>[2x]MYDWFSEMRKKDPVYYDGNIWQVFSYRYTKEVLNNFSKFSSDLTGYHERLEDLRNGKIRFDIPTRYTMLTSDPPLHDELRSMSADIFS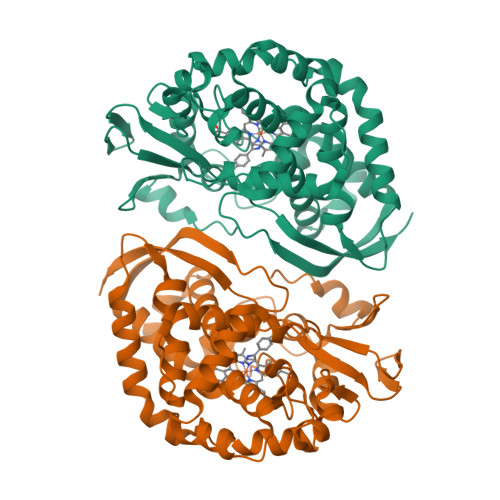PQKLQTLETFIRETTRSLLDSIDPREDDIVKKLAVPLPIIVISKILGLPIEDKEKFKEWSDLVAFRLGKPGEIFELGKKYLELIGYVKDHLNSGTEVVSRVVNSNLSDIEKLGYIILLLIAGNETTTNLISNSVIDFTRFNLWQRIREENLYLKAIEEALRYSPPVMRTVRKTKERVKLGDQTIEEGEYVRVWIASANRDEEVFHDGEKFIPDRNPNPHLSFGSGIHLCLGAPLARLEARIAIEEFSKRFRHIEILDTEKVPNEVLNGYKRLVVRLKSNE(5~{S},7~{R},8~{S},9~{S},10~{R})-7-(hydroxymethyl)-2-naphthalen-1-yl-8,9,10-tris(oxidanyl)-6-oxa-1,3-diazaspiro[4.5]dec-1-en-4-one | C18 H18 N2 O6 | 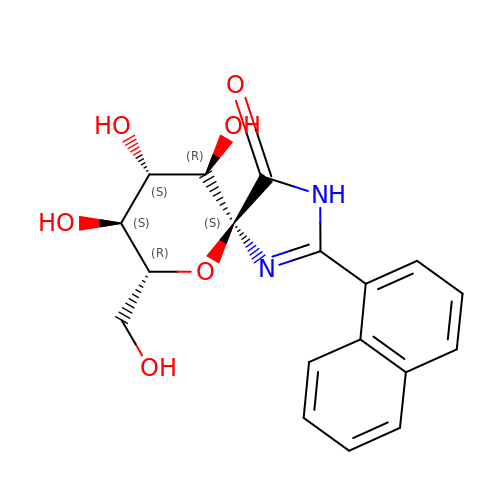VIYRJCLPOZQRSZ-NSIVTLKISA-N> GYDSILVQATPRKSS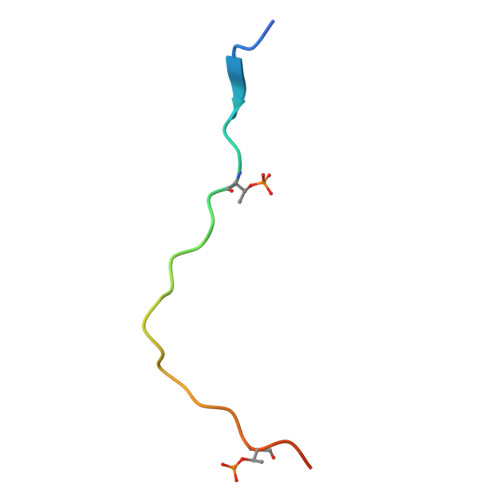SVITELPDTPIKMNS>[8x]AAASMSALITENMHMKLYMEGTVNNHHFKCTSEGEGKPYEGTQTMRIKVVEGGPLPFAFDILATSFMYGSKTFINHTQGIPDFFKQS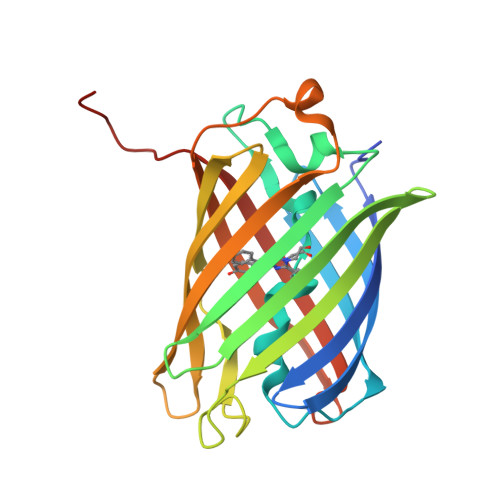FPEGFTWERVTTYEDGGVLTATQDTSLQDGCLIYNVKIRGVNFPSNGPVMQKKTLGWEACTEMLYPADGGLEGRADMALKLVGGGHLICNLKTTYRSKKPAKNLKMPGVYYVDRRLERIKEADKETYVEQHEVAVARYCDLPSKLAHK> DYKDDDDKLEVLFQGPGSLPVIAELPPKVSVFVPPRDGFFGNPRKSKLICQATGFSPRQIQVSWLREGKQVGSGVTTDQVQAEAKESGPTTYKVTSTLTIKESDWLGQSMFTCRVDHRGLTFQQNASSM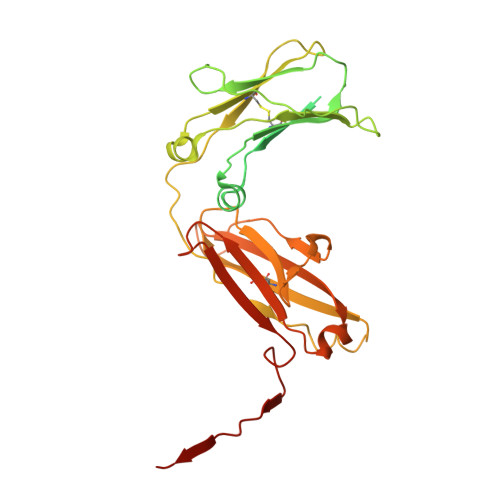CVPDQDTAIRVFAIPPSFASIFLTKSTKLTCLVTDLTTYDSVTISWTRQNGEAVKTHTNISESHPNATFSAVGEASICEDDWNSGERFTCTVTHTDLPSPLKQTISRPKGVALHRPDVYLLPPAREQLNLRESATITCLVTGFSPADVFVQWMQRGQPLSPEKYVTSAPMPEPQAPGRYFAHSILTVSEEEWNTGETYTCVVAHEALPNRVTERTVDKSTGKPTLYNVSLVMSDTAGTCY5,5'-(sulfanediyldiethane-2,1-diyl)bis(1,3,4-thiadiazol-2-amine) 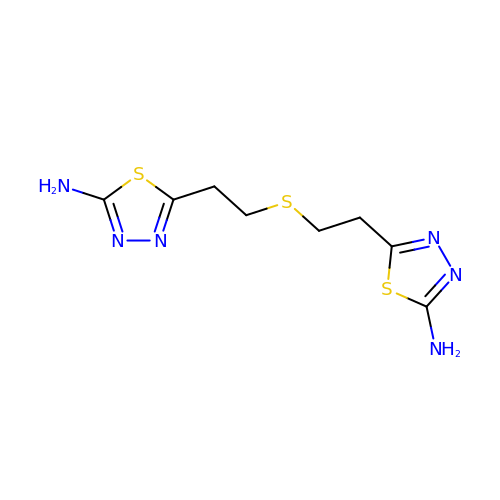| C8 H12 N6 S3 | AOAQKDDVWLOZFV-UHFFFAOYSA-N>[4x]SMTWLPLNPIPLKDRVSMIFLQYGQIDVIDGAFVLIDKTGIRTHIPVGSVACIMLEPGTRVSHAAVRLAAQVGTLLVWVGEAGVRVYASGQPGGARSDKLLYQAKLALDEDLRLKVVRKMFELRFGE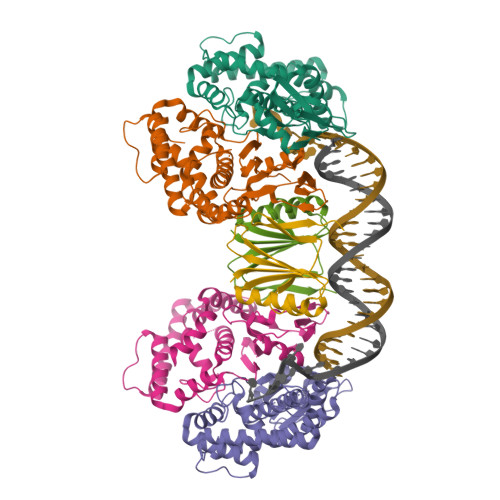PAPARRSVEQLRGIEGSRVRATYALLAKQYGVTWNGRRYDPKDWEKGDTINQCISAATSCLYGVTEAAILAAGYAPAIGFVHTGKPLSFVYDIADIIKFDTVVPKAFEIARRNPGEPDREVRLACRDIFRSSKTLAKLIPLIEDVLAAGEIQPPAPPEDAQPVAIPLPVSLGDAGHRSS;>MMSMLVVVTENVPPRLRGRLAIWLLEVRAGVYVGDVSAKIREMIWEQIAGLAEEGNVVMAWATNTETGFEFQTFGLNRRTPVDLDGLRLVSFLPVGSSENLYFQ[2x]> XADVAGTSNRDFRGREQRLYNSEQYNYNNSLNGEVSLWVYAYYSDGSVLVRNCNSQYKVGISECFKSLKEVRVGQNNDPYDEQEVNNGVYYPNGGEPTKFHSNAKPRAIQIIFSPSVNVHTIKMAKGNSVSIPKDYLQRSHPWEATGVKYRKIHVDGEIVGYSHYFELPHEYNSISLSVSGVHKNPSSYNVAAPHNIMDVFQSCDLALKFSNRYWCELELINHYISAYAYPYLDINNHKYGVPLNGRQ

Following this approach, we have developed a microchip from single crystalline silicon with a periodic structure of micropores that serves as sample holder for several thousand microcrystals. To prove the suitability of our chip for protein micro-crystallography, polyhedrin and lysozyme microcrystals of less than 4 μm in size were chosen as test samples for X-ray diffraction experiments. X-ray data collections from both protein crystals were performed at the microfocus beamline I24 at Diamond Light Source at a temperature of 100 K with a photon flux of ~2 × 1011 ph/sec and an X-ray beam size of a 7 × 7 μm2 (FWHM) at a photon energy of 12.8 keV. The use of single-crystalline silicon and the efficient removal of the mother liquor lead to exceptionally low background scattering caused by the chip.

The polyhedrin microcrystals diffracted to a high resolution of 1.5 Å. A total number of 51 datasets were collected at different positions on the chip of which 23 datasets could be indexed and 22 were merged into the final dataset. No obvious signs of radiation damage can be observed upon inspection of the Fo-Fc difference electron densities. Seleno-methionine labeled polyhedrin crystals are typically of lower quality and exhibit worse diffraction properties than their native counterparts. Thus, with similar data collection parameters, the higher resolution achieved in our experiment is very likely a consequence of the efficient removal of mother liquor and the use of single crystalline silicon as a low-background substrate for the chip. As a result diffraction data collected from seleno-methionine labeled polyhedrin microcrystals loaded onto our chip are of superior quality compared to diffraction data from conventionally mounted native crystals. The doses applied to the crystals, 28.5 MGy in case of polyhedrin and 20.2 MGy in case of lysozyme, are below the acceptable dose limits for cryocrystallography as reported in the literature. The structure determinations are based on measurements of 52 polyhedrin and 139 lysozyme microcrystals with sizes of 4 micrometer and smaller.>[2x]GAMEEKYLPELMAEKDSLDPSFTHALRLVNQEIEKFQKGEGKDEEKYIDVVINKNMKLGQKVLIPVKQFPKFNFVGKLLGPRGNSLKRLQEETLTKMSILGKGSMRDKAKEEELRKSGEAKYFHLNDDLHVLIEVFAPPAEAYARMGHALEEIKKFLIPDYNDEIRQAQLQELTYLNGGSENADV

T-STAR is a tissue-specific STAR protein mainly expressed in the testis and brain3426, and regulates the alternative splicing of CD44, Tra2β, Tau, VGEF and Neurexin pre-mRNAs262728. STAR proteins are defined by the presence of a highly conserved RNA-binding domain, the STAR domain, also responsible for homodimerization, and composed of a central KH (K homology) domain flanked by two highly conserved regions, QUA1 and QUA2. Here, we have determined the X-ray structures of the T-STAR KH domain in its free state, and in complex with AAAUAA; KH-QUA2 in complex with AAUAAU; QUA1-KH in complex with UAAU; and the full STAR domain in complex with AUUAAA. Taken together, our data reveal a unique mode of RNA recognition and dimerization by the STAR proteins Sam68 and T-STAR that is crucial for their function in alternative splicing.

The structures of the T-STAR QUA1-KH and STAR domains in complex with RNA show that the QUA1 and the KH domains form compact dimers, with each KH domain binding one RNA molecule, while the QUA2 domain does not adopt a fixed orientation. The QUA1 domain adopts a helix-turn-helix motif involved in homodimerization, and its fold is very similar to the structure of isolated Sam68 QUA1 reported previously (backbone root mean square deviation (RMSD) of 0.61 Å). No electron density could be observed for the N-terminal half of the linker connecting the QUA1 to the KH domain (residues 35–42), suggesting that this region is disordered, while the C-terminal half of the linker (residues 43–53) is well defined in the structures. Strikingly, no electron density could be observed for the QUA2 region of T-STAR in all our data sets, suggesting that the QUA2 region does not adopt a well-defined orientation. Accordingly, the structure of T-STAR STAR in complex with AUUAAA overlay very well with the structure of T-STAR QUA1-KH in complex with UAAU with a backbone RMSD of 0.9 Å for the QUA1-KH atoms. Interestingly, the presence of the QUA2 region in the STAR domains increases the radius of gyration and maximal dimensions both in the absence and presence of RNA. This is consistent with the QUA2 domain being flexibly attached to the QUA1-KH domain dimer, and may explain that no electron density is observed for the QUA2 domain in the crystal structures of the T-STAR STAR and KH-QUA2 domains. The absence of electron density for the QUA2 domain in our X-ray data sets suggests that the QUA2 domain of T-STAR does not contribute to RNA binding. The crystal structures of T-STAR QUA1-KH and STAR domains show that the QUA1 dimer contacts only one KH domain. From our NMR and SAXS data in solution, we conclude that the contacts between the QUA1 dimer and one KH domain observed in our X-ray structures are most probably due to crystal packing.>MDHDFLKGQGDARSVRHIAIPAHRGLITDRNGEPLAVSTPVTTLWANPKELMTAKERWPQLAAALGQDTKLFADRIEQNAEREFIYLVRGLTPEQGEGVIALKVP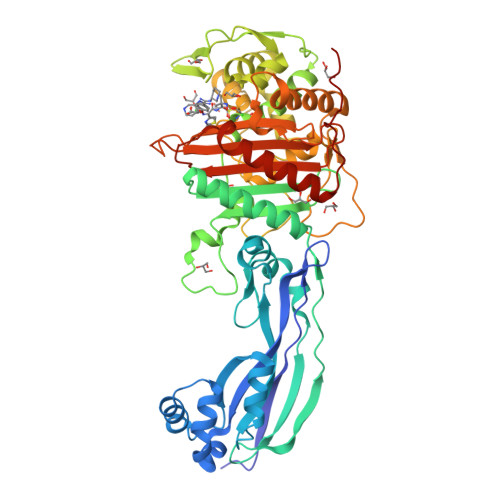GVYSIEEFRRFYPAGEVVAHAVGFTDVDDRGREGIELAFDEWLAGVPGKRQVLKDRRGRVIKDVQVTKNAKPGKTLALSIDLRLQYLAHRELRNALLENGAKAGSLVIMDVKTGEILAMTNQPTYNPNNRRNLQPAAMRNRAMIDVFEPGSTVKPFSMSAALASGRWKPSDIVDVYPGTLQIGRYTIRDVSRNSRQLDLTGILIKSSNVGISKIAFDIGAESIYSVMQQVGLGQDTGLGFPGERVGNLPNHRKWPKAETATLAYGYGLSVTAIQLAHAYAALANDGKSVPLSMTRVDRVPDGVQVISPEVASTVQGMLQQVVEAQGGVFRAQVPGYHAAGKSGTARKVSVGTKGYRENAYRSLFAGFAPATDPRIAMVVVIDEPSKAGYFGGLVSAPVFSKVMAGALRLMNVPPDNLPTAKLVPRG[2x]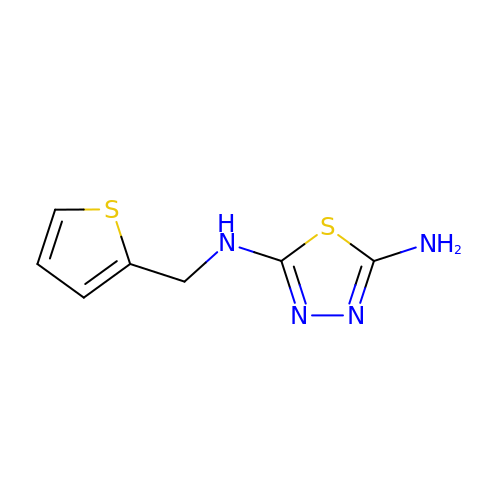N~2~-[(thiophen-2-yl)methyl]-1,3,4-thiadiazole-2,5-diamine | C7 H8 N4 S2 | KYOKGDLJKFUPBK-UHFFFAOYSA-N>[2x]MAHAGRTGYDNREIVMKYIHYKLSQRGYEWDAGDDVEENRTEAPEGTESEVVHLTLRQAVDDFSRRYRRDFAEMSSQLHLTPFTARGRFATVVEELFRDGVNWGRIVAFFEFGGVMCVESVNREMSPLVDNIALWMTEYLNRHLHTWIQDNGGWDAFVELYGPSMR

BCL-2 is the founding member of the pro-survival class of proteins that includes BCL-XL, BCL-W, A1/BFL-1 and MCL-1. They exert their pro-survival function by binding and restraining related members of a family of pro-apoptotic proteins—the sensors of cellular stress (the BH3-only proteins) and the effectors of apoptosis (BAX and BAK). Four or more hydrophobic amino acids on successive helical turns within the BH3 motif engage complementary pockets (P1 through P4) in this surface groove of pro-survival proteins. Venetoclax competes with pro-apoptotic BH3 motifs for BCL-2 binding, releasing pro-apoptotic proteins and allowing apoptosis in cells primed for death.

Recently a novel BCL-2 mutation was described exclusively in patients undergoing treatment with venetoclax. This mutant, G101V, was found in chronic lymphocytic leukaemia (CLL) patients from the clinical trials who had initially responded to treatment but developed CLL-type clinical progression after 19–42 months. The BCL-2 G101V mutation reduces the affinity for the drug to BCL-2 by some 180-fold. The BCL-2 G101V:venetoclax complex crystallised in P21 spacegroup with two molecules in the asymmetric unit diffracting to 2.2 Å, with well-defined electron density for both copies of the drug. The overall structure of BCL-2 G101V was similar to WT with no significant deviations in α2–α5 core helices or α6-α8. The binding pose of venetoclax is conserved between WT and the G101V mutant. Interestingly, the G101V mutation did not alter the positioning of the α2 helix relative to α5 or impact the residues defining the P4 pocket. Instead the additional bulk of the valine sidechain was accommodated by a deviation of the sidechains of Y18 on α1 and E152 on α5. In the BCL-2 G101V:venetoclax structure E152 had a 60º rotamer change relative to WT (mm-40 for WT to tp10 for G101V), placing the sidechain Cγ in van der Waal’s contact with the chlorine atom of the venetoclax chlorophenyl moiety. This conformational change in E152 in the BCL-2 G101V structure causes a small repositioning of the venetoclax 4DM and chlorophenyl moieties in the P2 pocket, moving on average 0.25 Å closer to L137 in the α4 helix, i.e. more similar to the BCL-2 WT complexes with ABT-263 and compound 1. Additionally, introduction of an alanine at the G101 position did not provide sufficient bulk to displace E152 in the crystal structure and affinity for venetoclax was maintained for the G101A mutant. Thus the functional consequences of the G101V mutant are felt in the P2 pocket via the ‘knock-on’ effect of E152 repositioning forced by the additional bulk of the valine sidechain.>[2x]GPELVMRRGEI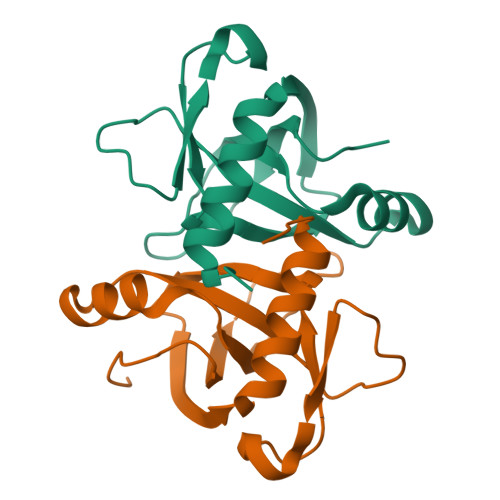WQVDLDPARGSEANNQRPAVVVSNDRANATATRLGRGVITVVPVTSNIAKVYPFQVLLSATTTGLQVDCKAQAEQIRSIATERLLRPIGRVSAAELAQLDEALKLHLDLWS Afamin is a human plasma glycoprotein and a member of the albumin gene family that has been reported to be a multifunctional transporter of hydrophobic molecules such as vitamin E and a potential binding partner for Wnt signalling proteins. The structural similarity of afamin to hSA suggests that afamin might also be able to transport cargo in the bloodstream. The availability of four independent afamin structure models from two different crystal forms provides insight into the flexibility and dynamics of the molecule, which point towards a significant conformational adaptability when binding to hydrophobic molecules, metal chelates or proteins with hydrophobic acylation such as Wnt, supporting the potential function of afamin as a promiscuous transport molecule in human plasma.

Here, we describe how the controlled dehydration of afamin crystals was able to stabilize a new orthorhombic crystal form, increasing the resolution, inducing a change in symmetry and increasing the number of intermolecular contacts, and leading to a more complete model. The use of a humidity-control device has allowed the orthorhombic crystal form to be stabilized. The transformation involves a contraction in the a cell edge of over 10 Å and of the β angle by ∼3°. The number of crystal contacts between symmetry-related molecules of <4 Å increases from 1999 to 2752 and the buried surface area increases from 968 to 1128 Å2. The result is a significant stabilization of the molecule that can be seen in the B factors. The possibility of forcing PEG molecules into binding sites as surrogate probes by dehydration is intriguing. In the example of afamin, the presence of the secondary binding channel occupied by a PEG molecule opens up the speculation that afamin could, at least from a structural point of view, also accommodate moieties with two fatty-acid chains, such as phosphatidylcholines.

> LPTQPRDIENFNSTQKFIEDNIEYITIIAFAQYVQEATFEEMEKLVKDMVEYKDRCMADKTLPECSKLPNNVLQEKICAMEGLPQKHNFSHCCSKVDAQRRLCFFYNKKSDVGFLPPFPTLDPEEKCQAYESNRESLLNHFLYEVARRNPFVFAPTLLTVAVHFEEVAKSCCEEQNKVNCLQTRAIPVTQYLKAFSSYQKHVCGALLKFGTKVVHFIYIAILSQKFPKIEFKELISLVEDVSSNYDGCCEGDVVQCIRDTSKVMNHICSKQDSISSKIKECCEKKIPERGQCIINSNKDDRPKDLSLREGKFTDSENVCQERDADPDTFFAKFTFEYSRRHPDLSIPELLRIVQIYKDLLRNCCNTENPPGCYRYAEDKFNETTEKSLKMVQQECKHFQNLGKDGLKYHYLIRLTKIAPQLSTEELVSLGEKMVTAFTTCCTLSEEFACVDNLADLVFGELCGVNENRTINPAVDHCCKTNFAFRRPCFESLKADKTYVPPPFSQDLFTFHADMCQSQNEELQRKTDRFLVNLVKLKHELTDEELQSLFTNFANVVDKCCKAESPEVCFNEESPKIGNKGENLYFQ> GSAENESTPIQQLLEHFLRQLQRKDPHGFFAFPVTDAIAPGYSMIIKHPMDFGTMKDKIVANEYKSVTEFKADFKLMCDNAMTYNRPDTVY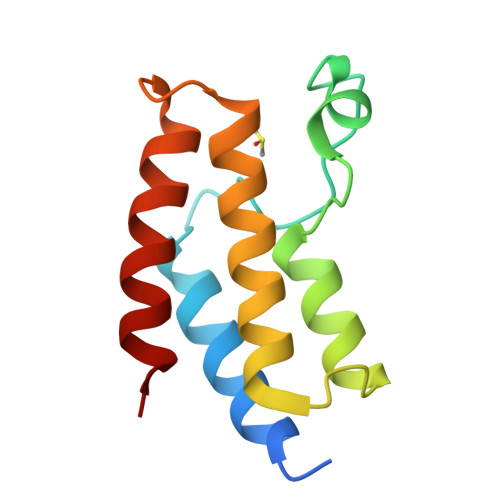YKLAKKILHAGFKMMSK2-phenylethyl 2-(4-azanyl-2-methanoyl-phenyl)ethanoate | C17 H17 N O3 | 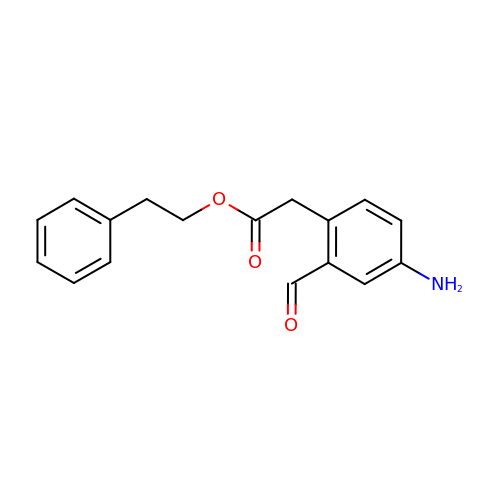VKURJRUODVXQJZ-UHFFFAOYSA-N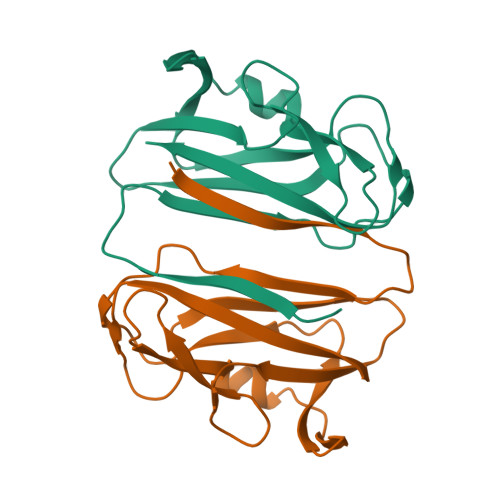>[2x]GSQKSVDIVFSSPQDLTVSLIPVSGLKAGKNAPSAKIAKLVVNSTTLKEFGVRGISNNVVDSTGTAWRVAGKNTGKEIGVGLSSDSLRRSDSTEKWNGVNWMTFNSNDTLDIVLTGPAQNVTADTYPITLDVVGYQP> SPDSAKISKEQLKKLHSNILNEIFSQSQVNKPGPLTVPF;> SMEAEKQSDIKGTIAFDTHGNVIESTGVGSQRIEDIGDLSKVTLDAEGFAQVQGDSLLVHLYKRNDITLAVYTSAQ;> MVMLHSKNVKGFLENTLKPYDLHSVDFKTSSLQSSMIITATNGGILSYATSNNDVPKNSINEINSVNNLKMMSLLIKDKWSEDENDTEEQHSNSCYPVEIDSFKTKIYTYEMEDLHTCVAQI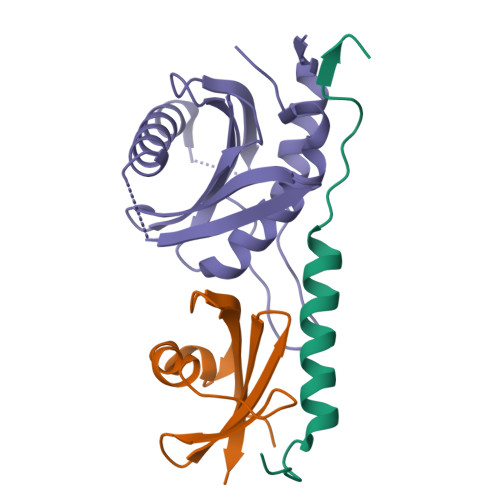PNSDLLLLFIAEGSFPYGLLVIKIERAMRELTDLFGYKLG>MRENKIIMISGANSGIGHACIKYFLEKSFHVIALDINNNNLIDYMKTDMPLKVVQIDLSNSEAIHNLFTQ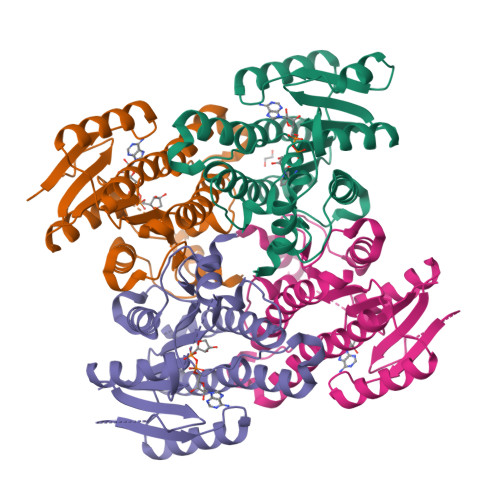LDLEKLSPDILINAAGIREITPVLHLSDDMFKKVIDVNLVAPFILSREVAKRWCESKIKGCIVNIASVSGLMAEPERAAYVASKHALIGLTKQMAMEFGKQNIRVNSISPGVIRTELTEEYFSNKALMSMIKSNQSLDTWGLPQDIVSCIEYLISDQARFITGSNFVIDGGWTAGKNLLEKGELNSKLEGKPIPNPLLGLDSTRTGHHHHHH[4x]2-(2-~{tert}-butylphenoxy)-~{N}-(4-hydroxyphenyl)ethanamide 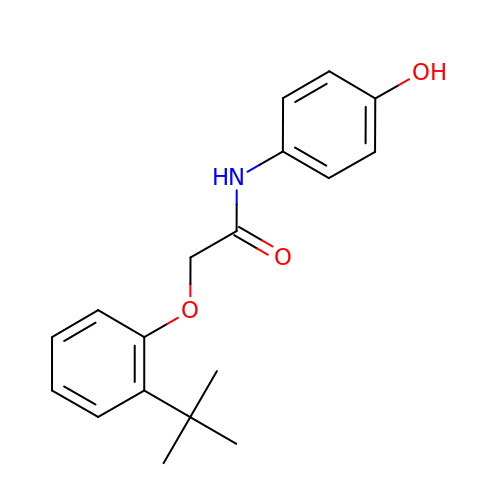| C18 H21 N O3 | RUNXUUCDTNJFME-UHFFFAOYSA-N Modulation of voltage-gated potassium (Kv) channels by auxiliary subunits is central to the physiological function of channels in the brain and heart. Native Kv4 tetrameric channels form macromolecular ternary complexes with two auxiliary β-subunits—intracellular Kv channel-interacting proteins (KChIPs) and transmembrane dipeptidyl peptidase-related proteins (DPPs)—to evoke rapidly activating and inactivating A-type currents, which prevent the backpropagation of action potentials. Here we report cryo-electron microscopy structures of the Kv4.2–DPP6S–KChIP1 dodecamer complex, the Kv4.2–KChIP1 and Kv4.2–DPP6S octamer complexes, and Kv4.2 alone. Thus, our data suggest that two distinct modes of modulation contribute in an additive manner to evoke A-type currents from the native Kv4 macromolecular complex.

The structure of the Kv4.2–KChIP1 complex reveals that the intracellular N terminus of Kv4.2 interacts with its C terminus that extends from the S6 gating helix of the neighbouring Kv4.2 subunit. KChIP1 captures both the N and the C terminus of Kv4.2. In consequence, KChIP1 would prevent N-type inactivation and stabilize the S6 conformation to modulate gating of the S6 helices within the tetramer. The present structure of the full-length Kv4.2–KChIP1 complex reveals that the C terminus of Kv4.2 tightly interacts with both KChIP1 and the N terminus of Kv4.2. The C-terminal cytoplasmic S6 helix continuously extends from the transmembrane S6 helix and terminates at S450, which is localized at the bottom of the complex. Although the residues from G451 to G471 are disordered, the following second cytoplasmic helix with a short loop (C-terminal segment: S472–D495) fits into the hydrophobic crevice formed by KChIP1 and the Kv4.2 N-terminal segment (A2–R35) from the neighbouring Kv4.2 subunit. In addition, the cytoplasmic S6 helix (around S450) is captured by KChIP1 directly and indirectly, through the hydrophobic interactions between Kv4.2 (Y444), Kv4.2 (H479-L482-F493) and KChIP1 (H84) and the electrostatic interactions of Kv4.2 (Y444–K448) with Kv4.2 (H483–E486), respectively. In the Kv4.2–KChIP1 complex, KChIP1s bind and sequester the both N-terminal inactivation ball and the C terminus (amino acids 472–495) of Kv4.2, which would therefore result in preventing N-type inactivation. Moreover, while S6 gating helices adopt a more flexible conformation with weaker interaction with T1–S1 linkers in the structure of Kv4.2 alone, KChIP1 stabilizes these structures and enhances their interactions in the structure of Kv4.2–KChIP1.

>MAAGVAAWLPFARAAAIGWMPVASGPMPAPPRQERKRTQDALIVLNVSGTRFQTWQDTLERYPDTLLGSSERDFFYHPETQQYFFDRDPDIFRHILNFYRTGKLHYPRHECISAYDEELAFFGLIPEIIGDCCYEEYKDRRRENAERLQDDADTDTAGESALPTMTARQRVWRAFENPHTSTMALVFYYVTGFFIAVSVIANVVETVPCGSSPGHIKELPCGERYAVAFFCLDTACVMIFTVEYLLRLAAAPSRYRFVRSVMSIIDVVAILPYYIGLVMTDNEDVSGAFVTLRVFRVFRIFKFSRHSQGLRILGYTLKSCASELGFLLFSLTMAIIIFATVMFYAEKGSSASKFTSIPAAFWYTIVTMTTLGYGDMVPKTIAGKIFGSICSLSGVLVIALPVPVIVSNFSRIYHQNQRADKRRAQKKARLARIRAAKSGSANAYMQSKRSGLLSNQLQSSEDEPAFVSKSGSSFETQHHHLLHCLEKTTNHEFVDEQVFEESCMEVATVNRPSSHSPSLSSQQGVTSTCCSRRHKKTFRIPNANVSGSHRGSVQELSTIQIRCVERTPLSNSRSSLNAKMEECVKLNCEQPYVTTAIISIPTPPVTTPEGDDRPESPEYSGGNIVRVSAL[4x];>[4x]MGAVMGTFSSLQTKQRRPSKDKIEDELEMTMVCHRPEGLEQLEAQTNFTKRELQVLYRGFKNECPSGVVNEDTFKQIYAQFFPHGDASTYAHYLFNAFDTTQTGSVKFEDFVTALSILLRGTVHEKLRWTFNLYDINKDGYINKEEMMDIVKAIYDMMGKYTYPVLKEDTPRQHVDVFFQKMDKNKDGIVTLDEFLESCQEDDNIMRSLQLFQNVM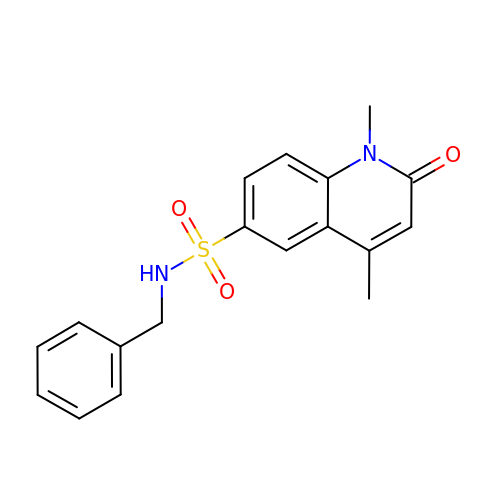1,4-dimethyl-2-oxidanylidene-~{N}-(phenylmethyl)quinoline-6-sulfonamide | C18 H18 N2 O3 S | KBXRBUMRPUNHEH-UHFFFAOYSA-N>TATGDEWWAKCKQVDVLDSEMSYYDSDPGKHKNTVIFLHGNPTSSYLWRNVIPHVEPLARCLAPDLIGMGKSGKLPNHSYRFVDHYRYLSAWF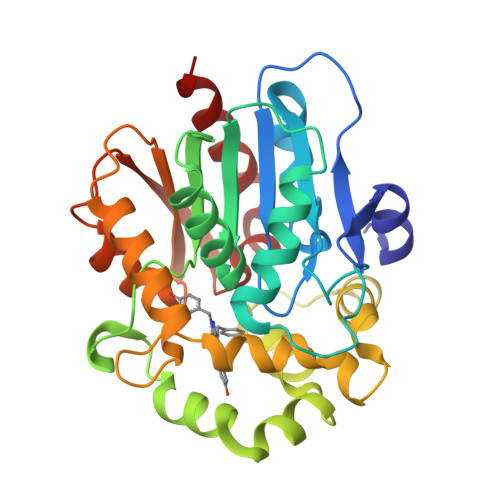DSVNLPEKVTIVCHDWGSGLGFHWCNEHRDRVKGIVHMESVVDVIESWDEWPDIEEDIALIKSEAGEEMVLKKNFFIERLLPSSIMRKLSEEEMDAYREPFVEPGESRRPTLTWPREIPIKGDGPEDVIEIVKSYNKWLSTSKDIPKLFINADPGFFSNAIKKVTKNWPNQKTVTVKGLHFLQEDSPEEIGEAIADFLNELT[3x]>HHHHHHSSGLVPRGSHMASQVVRIVGVGRTGIGKLHKSVDELAASALKCALVDANMKQCDLQALIAVPSLASPQFMQAHHIATVAGLFPTKGKFIVRTVDTGGAGPITALGMAVDLVRTRCAETVAVIAADAVLSMGSGAFAERSNASLRRSGLPEPCIPHGYDRYAQWYMSRYGLKREQLAMVPVLMSKMAERHPEAMCQKAYTLDEVLHSRCVAPVTNLLECARRADGAVALIVSGEAHYAEHFAQGKQEQRHLGGSKPIIASVAEASGPLFPPGSSDDIVPDIFSCRHAARDAFLSANLNVGDIHF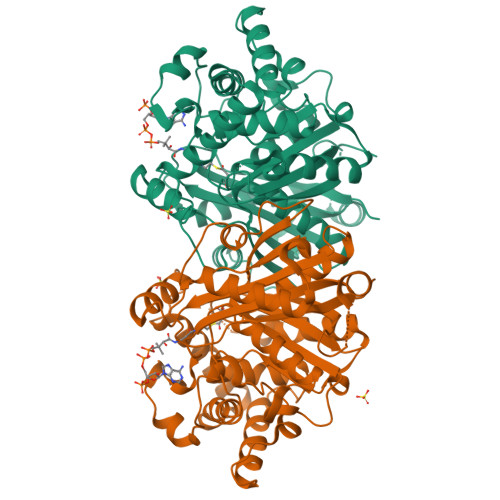FGLYDCFPICLIQAVEAVGLCPEGKGGEFMETAYNEMLNNGGVLDPSKFPINTHGGLQCFGAPWEVPAMYNITEAIAQLSEEAGDRQLTPVPKRALVYGNGGIFSASSVAILISDL[6x]>MSKSLQLIKEHDVKWIDLRFTDTKGKQQHVTMPARDVDDDFFEYGKMFDGSSIAGWKGIEASDMILMPDDSTAVLDPFTEEPTLIIVCDIIEPSTMQGYDRDPRAIARRAEEYLKSTGIGDTAFFGPEPEFFIFDEVKYKSDISGSMFKIFSEQAAWNTDADFEGGNKGHRPGVKGGYFPVPPVDHDHEIRTAMCNALEEMGLKVEVHHHEVATAGQNEIGVSFNTLVAKADEVQTLKYCVHNVADAYGKTVTFMPKPLYGDNGSGMHVHMSIAKDGKNTFAGEGYAGLSDTALYFIGGIIKHGKALNGFTNPSTNSYKRL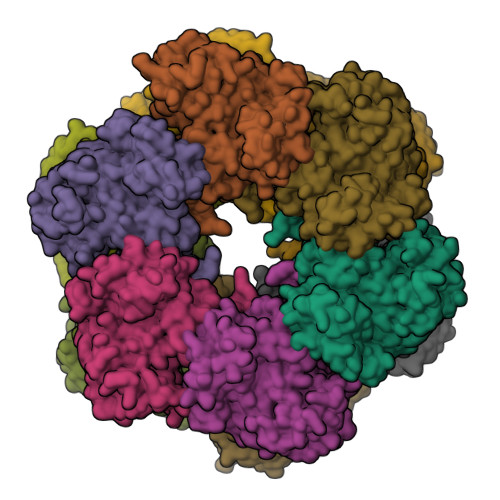VPGFEAPVMLAYSARNRSASIRIPYVNSPKARRIEARFPDPSANPYLAFAALLMAGLDGIQNKIHPGDAADKNLYDLPPEEAKEIPQVCGSLKEALEELDKGRAFLTKGGVFSDDFIDAYLELKSEEEIKVRTFVHPLEYDLYYSV[12x]(2S)-2,3-dihydroxy-2-methylpropanoic acid | C4 H8 O4 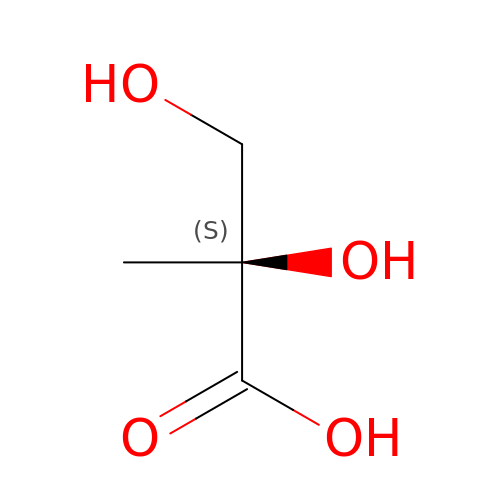| DGADNPLBVRLJGD-BYPYZUCNSA-N> MGAHASVIKPEMKIKLRMEGAVNGHKFVIEGEGIGKPYEGTQTLDLTVEEGAPLPFSYDILTPAFXNRAFTKYPEDIPDYFKQAFPEGYSWERSMTYEDQGICIATSDITMEGDCFFYEIRFDGTNFPPNGPVMQKKTLKLIDATEKM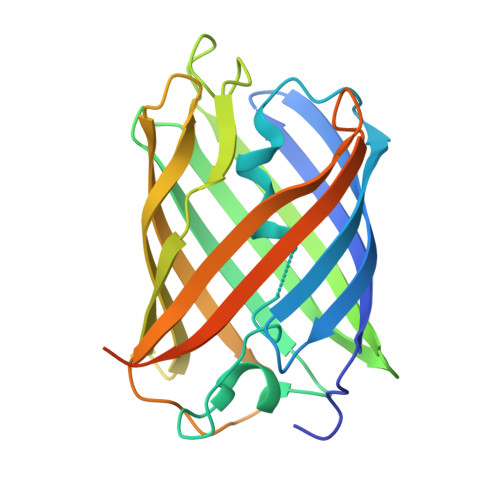YVEDGVLKGDVEMALLLEGGGHYRCDFKTTYKAKKDVRLPDAHEVDHRTEILKHDKDYNKVRLYEHAEARYSGGGSGGGASGKPIPNPLLGLDSTHHHHHH>[3x]GMEQLQKRKIYDTTASNASTGILNGKSSNVLNWDDVRFSWAYPLYKNMLANFWTPFEINMSHDAKQFPTLTETEQEAFKKIIGLLAFLDSVQTDYSMRAAEYLTDSSLAALMSVLSFQEVVHNQSYSYVLSSLVPKATQDEIFEYWKHDDVLKERNEFIIDGYEKFVDNPTPKTFLESIVYDVILEGLNFYSGFAFFYNLARNQKMVSTSTMINYINRDEQLHVYLFTNIFKELLVEFPEL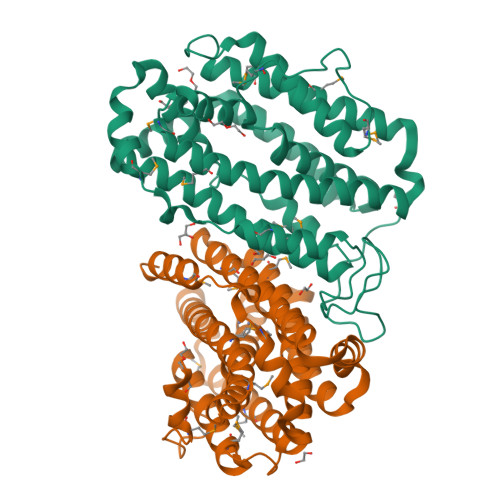NTEETKTFVKTTLMKAADLEKDWFRYIIGDKIPGINPEDMETYISFIANKRAVQLGMEKPYPEIKHNPMKWIRAYEDVNSGKSDFFEQKSRQYAKVSADNGFDEL Mitochondrial Hsp60 (mtHsp60) plays a crucial role in maintaining the proper folding of proteins in the mitochondria. mtHsp60 self-assembles into a ring-shaped heptamer, which can further form a double-ring tetradecamer in the presence of ATP and mtHsp10. The crystal structure of mtHsp60 reveals three domains: apical, intermediate, and equatorial domains. The equatorial domain connects the subunits in the heptameric ring and facilitates interactions between the two rings of tetradecamers. Our results showed that the E. coioides mtHsp60 (EcHsp60) forms dimers that are incapable of hydrolyzing ATP but can reassemble into heptamers, thus restoring ATPase activity.

As an alternative, we truncated the highly dynamic C-terminal GGM repeats of naïve EcHsp60 (Δ527–552), based on the crystallographic study of human mtHsp60. The resulting truncated protein, called naïve EcHsp60ΔC, was purified as a stable heptameric complex at both 4°C and RT. Importantly, the heptameric naïve EcHsp60ΔC showed similar ATPase activity to the WT naïve EcHsp607, indicating that the C-terminal truncation did not significantly affect the protein structure. The crystal structure of naïve EcHsp607 showed a typical heptameric, single-ring conformation in an asymmetric unit. Unlike the partially disordered equatorial domain of naïve EcHsp602, most regions of naïve EcHsp607 could be observed in the electron density maps, except for the N-terminal MIS and two C-terminal residues (residues 525–526). The β1/β16 strands form a strong interaction with the β2/β3 strands of the neighboring protomer and stabilize the heptameric complex. The thermal parameter distribution of the naïve EcHsp607 coordinate showed relatively low b-factor values in the equatorial domain compared with the apical and intermediate domains, suggesting that the equatorial domain is stabilized upon forming the heptameric conformation. The α4 helix of naïve EcHsp607 was found to be folded into the core region of the equatorial domain with α1, α5, α16, and α20, whereas in naïve EcHsp602, the α4 helix extended out from the equatorial domain and interacts with the neighboring subunit. In naïve EcHsp607, the ATP-binding motif, DGTTT, is located in the N-terminus of α4 helix and forms a pocket with G414 and D494.

>MFRLPTVMKQVRPVCRALAPHLTRAYAKDVKFGADARALMLQGVDLLADAVAVTMGPKGRTVIIEQSWGSPKVTKDGVTVAKSIDLKDKYKNIGAKLVQDVANNTNEEAGDGTTTATVLARAIAKEGFDTISKGANPVEIRRGVMMAVETVIKELKNLSKPVTTPEEIAQVATISANGDVEIGNIISNAMKKVGRKGVITVKDGKTLHDELEIIEGMKFDRGYISPYFINTAKGQKCEFQDAYLLLSEKKISSVQSIVPALEIANQHRKPLVIVAEDVDGEALSTLVLNRLKVGLQVVAVKAPGFGDNRKNQLRDMAVATGGTVFGDEAVGLALEDIQAHDFGKIGEVQITKDDTLLLKGGGSPAEVEKRAAEIVEQLENTTSDYEKEKLNERLAKLSDGVAVLKVGGTSDVEVNEKKDRVTDALNATRAAVEEGIVPGGGCALLRCIPSLDAIQTANADQKIGVEIIRRALRIPAMTIAKNAGVEGSLVVEKILQGSAELGYDAMQGEYVNMVEKGIIDPTKVVRTALLDAAGVASLLSTAEAVVTEIPKEDIHMFRLPTGMGFLEHHHHHH[7x]>VSEDLRSRIEVLKRKVIEKVQHIQLLQKNVRAQLVDMKRLEVDIDIKIRSCRGSCSRALAREVDLKDYEDQQKQLEQVIAKDLLPSR[2x];>DNENVVNEYSSELEKHQLYIDETVNSNIPTNLRVLRSILENLRSKIQKLESDVSAQMEYCRTPCTVSCNIPVVSGKECEEIIRKGGETSEMYLIQPDSSVKPYRVYCDMNTENGGWTVIQNRQDGSVDFGRKWDPYKQGFGNVATNTDGKNYCGLPGEYWLGNDKISQLTRMGPTELLIEMEDWKGDKVKAHYGGFTVQNEANKYQISVNKYRGTAGNALMDGASQLMGENRTMTIHNGMFFSTYDRDNDGWLTSDPRKQCSKEDGGGWWYNRCHAANPNGRYYWGGQYTWDMAKHGTDDGVVWMNWKGSWYSMRKMSMKIRPFFPQQ[2x];>KMLEEIMKYEASILTHDSSIRYLQEIYNS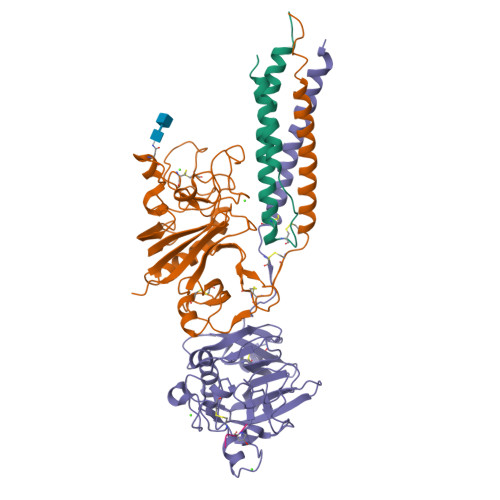NNQKIVNLKEKVAQLEAQCQEPCKDTVQIHDITGKDCQDIANKGAKQSGLYFIKPLKANQQFLVYCEIDGSGNGWTVFQKRLDGSVDFKKNWIQYKEGFGHLSPTGTTEFWLGNEKIHLISTQSAIPYALRVELEDWNGRTSTADYAMFKVGPEADKYRLTYAYFAGGDAGDAFDGFDFGDDPSDKFFTSHNGMQFSTWDNDNDKFEGNCAEQDGSGWWMNKCHAGHLNGVYYQGGTYSKASTPNGYDNGIIWATWKTRWYSMKKTTMKIIPFNRLTIGEGQQHHLGGAKQAGDV[2x];>[2x]GPRPX> MFADRLFNAMERNEPAPGMVLVAAPSMESEDFARSVILIIEHSEYATFGVNLASRSDVAVFNVIPEWVPCVTKPQALYIGGPLNQQSVVGVGVTAQGVDAARVDNLTRLA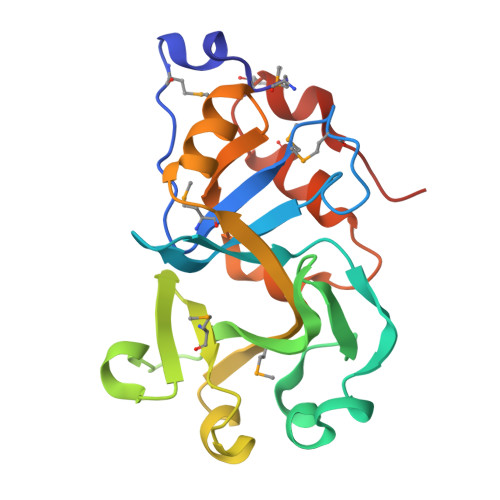NRLVMVNLGADPEEIKPLVSGMRLFAGHAEWAPGQLAQEIENGDWFVAPALPSDVTAPGSVDVWGDVMRRQPMPLPLYSTFPVNVGEN>SDKPVAHVVANHQVEEQLEWLSQRANALLANGMDLKDNQLVVPADGLYLVYSQVLFKGQGCPDYVLLTHTVSRFAISYQEKVNLLSAVKSPCPKDTPEGAELKPWYEPIYLGGVFQLEKGDQLSAEVNLPKYLDFAESGQVYFGVIAL[3x];>GSVCPQGKYIHPQDNSICCTKCHKGTYLYNDCPGPGQDTDCRECESGSFTASENHLRHCLSCSKCRKEMGQVEISSCTVDRDTVCGCRKNQYRHYWSENLFQCFNCSLCLNGTVHLSCQEKQNTVCTCHAGFFLRENECVSSSN[3x]

TNF, like most members of the TNF superfamily (TNFSF) exists mainly as a trimer with a threefold symmetry resulting in three identical receptor binding sites. The mechanism by which TNF induces signalling across the membrane is poorly understood, however, it is generally believed that the process involves receptor clustering. There are currently five approved TNF biologics that work by completely blocking the interaction of TNF with its receptors but to date, there are no small molecule therapeutics available that disrupt the high-affinity TNF–TNFR interaction. Small molecule inhibitors of TNF are described that stabilise a distorted TNF trimer, reducing the affinity of TNFR1 at one binding site and effectively reducing the stoichiometry of receptor binding from three to two per TNF trimer.

In order to further understand the impact of our compounds on receptor binding, we have crystallised mTNF with and without compound (UCB-4433) in complex with a truncated form of hTNFR1 (residues 41–184). All attempts to crystallise the complex made with a more complete receptor (residues 41–201) failed as did attempts to crystallise a complex of human TNF with humanTNFR1 regardless of the receptor length. In order to highlight the degree of distortion of the, arbitrarily defined, A–C receptor binding site, the UCB-4433 bound mTNF–hTNFR1 structure was compared with the complex without compound by aligning them through monomer C. There were no structural clashes within the long-form receptor dimer and only a minor clash between receptor and TNF suggesting that such a complex could form with only very minor changes in the receptor. In the overlay, the CRD4s within the receptor dimers were well separated (highlighted in red at the bottom of each dimer pair), suggesting that a significant conformational change would be needed if they were to form any kind of direct contact, so it is probable that the long-form receptor dimer present in signalling networks has an alternative conformation to that shown.>MAEQVLPQALYLSNMRKAVKIRERTPEDIFKPTNGIIHHFKTMHRYTLEMFRTCQFCPQFREIIHKALIDRNIQATLESQKKLNWCREVRKLVALKTNGDGNCLMHATSQYMWGVQDTDLVLRKALFSTLKETDTRNFKFRWQLESLKSQEFVETGLCYDTRNWNDEWDNLIKMASTDTPMARSGLQYNSLEEIHIFVLCNILRRPIIVISDKMLRSLESGSNFAPLKVGGIYLPLHWPAQECYRYPIVLGYDSHHFVPLVTLKDSGPEIRAVPLVNRDRGRFEDLKVHFLTDPENEMKEKLLKEYLMVIEIPVQGWDHGTTHLINAAKLDEANLPKEI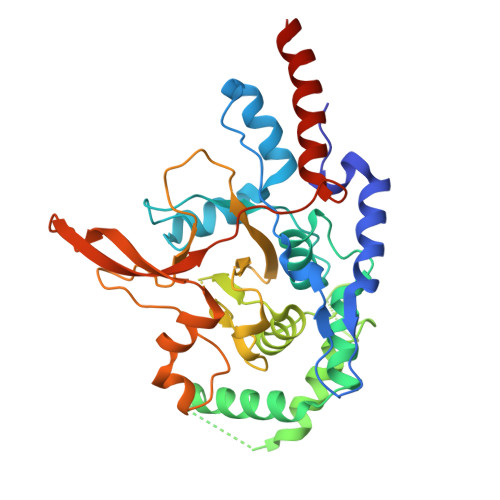NLVDDYFELVQHEYKKWQENSEQGRRE[4x]> TEPTIHKGLAGVTADVTAISKVNSDTNSLLYRGYPVQELAAKCSFEQVAYLLWNSELPNDSELKAFVNFERSHRKLDENVKGAIDLLSTACHPMDVARTAVSVLGANHARAQDSSPEANLEKAMSLLATFPSVVAYDQRRRRGEELIEPREDLDYSANFLWMTFGEEAAPEVVEAFNVSMILYAEHSFNASTFTARVITSTLADLHSAVTGAIGALKGPLHGGANEAVMHTFEEIGIRKDESLDE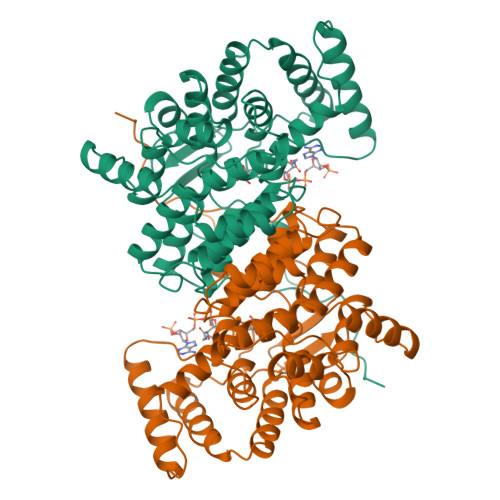AATRSKAWMVDALAQKKKVMGFGHRVYKNGDSRVPTMKSALDAMIKHYDRPEMLGLYNGLEAAMEEAKQIKPNLDYPAGPTYNLMGFDTEMFTPLFIAARITGWTAHIMEQVADNALIRPLSEYNGPEQRQVP Opioid-binding protein cell-adhesion molecule like (OPCML) is a glycosylphosphatidylinositol (GPI)-anchored protein that localizes to the outer leaflet of the plasma membrane and acts as a tumor suppressor (TS). OPCML consists of three Ig-like domains termed D1, D2, and D3, connected by short extended linkers. OPCML is composed of three canonical Ig-like domains with a C-terminal GPI anchor localized in the plasma membrane outer leaflet. We previously reported that OPCML interacts with a subset of RTKs and induces their degradation and/or dephosphorylation when re-expressed in ovarian cancer cells.

To localize the clinical mutations on the three-dimensional structure of OPCML and to gain insights into their role in the tumor suppressor mechanism(s) we crystallized soluble recombinant OPCML (residues 36–316) and determined its structure using a combined single-wavelength X-ray anomalous dispersion/molecular replacement approach. Structure solution was complicated initially by a high degree of translational pseudosymmetry, but identification of the correct space group and non-crystallographic symmetry elements allowed for chain tracing, which was followed by rounds of automated and manual model building and refinement. The OPCML homodimer resembles an inverted V shape, with dimerization mediated by a membrane-distal D1-D1 interface stabilized by a combination of hydrophobic contacts, hydrogen bonds and salt bridges. This interface comprises 874 Å2 of buried surface area and has a solvation free energy gain (ΔiG) on formation calculated by PISA to be −9.5 kcal M−1. The OPCML dimer is stabilized by reciprocal salt bridges between Arg 65 of one monomer and Asp 80 of the other. Below this lies a network of mainly hydrophobic contacts mediated by the stacking of Trp 82, Ile 74, Leu 69, Thr 114 and Arg 127. Overall, the D1-D1 dimerization interface is highly conserved since five of the seven key residues at the interface are absolutely conserved across the IgLON family (i.e. Leu 69, Ile 74, Asp 80, Trp 82, and Thr 114), with conservative substitutions at the other positions (Arg 65 is Lys in LSAMP and NEGR1 and Arg 127 is Gln in LSAMP, IGLON5, and NEGR1). Well-ordered glycans were observed at each Asn 70 in the crystal structure, allowing modelling of NAG-NAG-MAN glycosylation sequences. Asn 70 and the first NAG residue are completely buried by D1 and lie close to, but do not make specific contacts with, the reciprocal D1.

>ATFPKAMDNVTVRQGESATLRCTIDDRVTRVAWLNRSTILYAGNDKWSIDPRVIILVNTPTQYSIMIQNVDVYDEGPYTCSVQTDNHPKTSRVHLIVQVPPQIMNISSDITVNEGSSVTLLCLAIGRPEPTVTWRHLSVKEGQGFVSEDEYLEISDIKRDQSGEYECSALNDVAAPDVRKVKITVNYPPYISKAKNTGVSVGQKGILSCEASAVPMAEFQWFKEETRLATGLDGMRIENKGRMSTLTFFNVSEKDYGNYTCVATNKLGNTNASITLYGPGAALVPR[2x]>[2x]MAHHHHHHMDPQSTAAATVLKRAVELDSESRYPQALVCYQEGID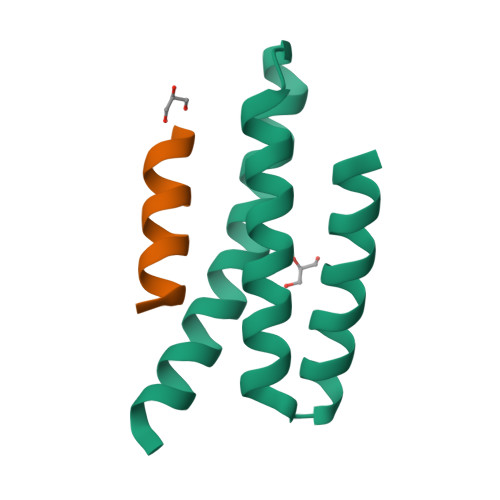LLLQVLKGTKDNTKRCNLREKISKYMDRAENIKKYLDQEKED;>[2x]SHMEDQLSRRLAALRN> MSHTDLTPCTRVLASSGTVPIAEELLARVLEPYSCKGCRYLIDAQYSATEDSVLAYGNFTIGESAYIRSTGHFNAVELILCFNQLAYSAFAPAVLNEEIRVLRGWSIDDYCQHQLSSMLIRKASSRFRKPLNPQKFSARLLCRDLQVIERTWRYLKVPCVIEFWDENGGAASGE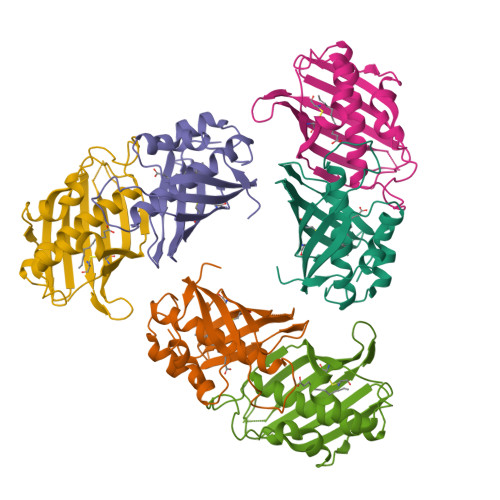IELAALNIP> LEEHYYSRKTCGSGGGLSVQRTGYPQTDPPVFKAVNSFERAPLIVGDHVHSLPYWSRKITLECTPYPFTLRWEGGVHKDGIPDKVPHPSCDPGSELVSYTHSREVDCERFIG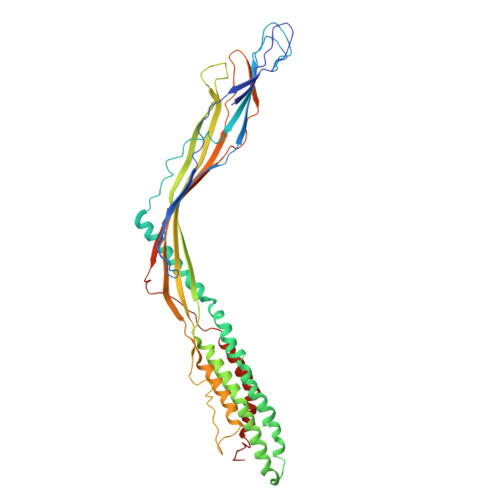PVPSSFTDPKVTSAQWKFLEDMADMKALADLNKSLVNLPMLYKERRETLKMVGNRLGGLVRVAHAAQDRDLKRYFKARRKDRRKVAEEVANGHLELIFGWLPLIGELEGAIEYAELPDLDFIRCHGLHTLVLQSTPWDNSVDVRSYPNWERAAGTRITGSVRTRGVVESRASVRTALRFNLETSLAGDARRLGFEPISTTYDMIPLSFVVGWFSNFDKYVRTLAPLIGVTFETGSQNRRTTCELVGCTRFYPRTVSPPSGWFARWKDFPDGSLSEVSGLRRTDIRSVLSTLPDPDVRFHADVGLFEISAGISLLAQRYLKPLQRLLKRKSFFYGRT> GDVQNAVEGAMVRVADTVQTSATNSERVPNLTAVETGHTSQAVPGDTMQTRHVINNHVRSESTIENFLARSACVFYLEYKTGTKEDSNSFNNWVITTRRVAQL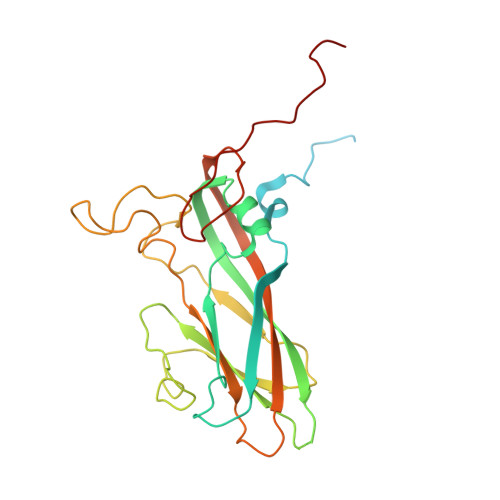RRKLEMFTYLRFDMEITVVITSSQDQSTSQNQNAPVLTHQIMYVPPGGPIPVSVDDYSWQTSTNPSIFWTEGNAPARMSIPFISIGNAYSNFYDGWSHFSQAGVYGFTTLNNMGQLFFRHVNKPNPAAITSVARIYFKPKHVRAWVPRPPRLCPYINSTNVNFEPKPVTEVRTNIITT>[2x]GIDPFTARPSSSMADFRKFFAKAKHIVIISGAGVSAESGVPTFRGAGGYWRKWQAQDLATPLAFAHNPSRVWEFYHYRREVMGSKEPNAGHRAIAECETRLGKQGRRVVVITQNIDELHRKAGTKNLLEIHGSLFKTRCTSCGVVAENYKSPICPALSGKGAPEPGTQDASIPVEKLPRCEEAGCGGLLRPHVVWFGENLDPAILEEVDRELAHCDLCLVVGTSSVVYPAAMFAPQVAARGVPVAEFNTETTPATNRFRFHFQGPCGTTLPEALA

Sirtuins are protein deacetylases and hydrolyze one NAD+ for each Lys residue they deacetylate, which links their activity to cellular energy levels. The conserved Sirtuin catalytic core comprises a Rossmann fold domain and a Zn2+-binding domain. The substrate polypeptide occupies a cleft between these domains, with the acetyl-Lys in a tunnel leading to the active site. Here, we show that resveratrol can directly activate the deacetylase activity of Sirt5 and inhibit the enzyme’s desuccinylase function as well as Sirt3-dependent deacetylation.

To rationalize the mechanism of Sirt5 activation in the FdL assay, we solved a crystal structure of Sirt5 in complex with FdL1 substrate peptide and resveratrol. Data quality was impaired by significant twinning (twin fraction 47%), and the density for resveratrol further weakened by its low occupancy (∼50%), likely due to its low solubility. However, density not accounted for by the built Sirt5/FdL1 model indicated an activator molecule bound close to the peptide substrate, directly contacting the FdL fluorophore. In the Sirt5/FdL1-peptide/resveratrol structure, the asymmetric unit contains two Sirt5 monomers with the active centers facing each other. Due to limited space resulting from this orientation only one peptide binding cleft is occupied by FdL1-peptide. The acetyl-Lys points toward the catalytic His158, and the FdL1 N-terminus occupies the same peptide binding channel as observed in other Sirtuin/peptide complexes. The C-terminal FdL1 fluorophore is packed with one surface on top of a hydrophobic patch formed by Tyr255 and Pro256 in the β7/α11 loop, and its edge is approached by Arg71. The activator A-ring is bound between Thr278 and Thr279 in the β8/α13 loop on one side, and Gly72 and Ala73 in the α2/α3 loop on the other side. The resveratrol B-ring interacts in almost perpendicular orientation with the coumarin fluorophore and contacts a protein patch formed by Gln83 and the α2/α3 loop around Arg71 and Gly72. The structure indicates that binding of resveratrol between the α2/α3 and β8/α13 loops closes the active site opening, thereby trapping the bound peptide and increasing the interaction interface by directly contacting the FdL1 substrate fluorophore.> MAEHRIPVLLLLVVVAASSLAQQIPLQKHYIIYEVRNIEKTPEEVKEEMKDTDILYSFKALGAPSYHIVVEVNPRNMRKLEEVELKGKIRMVPVVNMVDVAETLGVSWPRSGARLLDVNLTLIERTLNQEGLTSQESEAHLKGFMEELKDRLQQYNYQAFFTIGASPPKMYI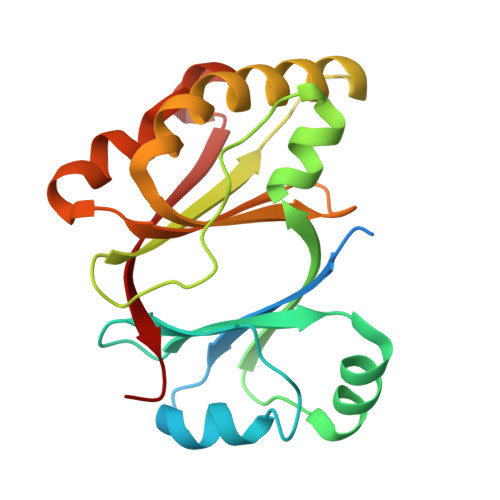YINIPYEEVDKFACIGINQFGGPAAVNTTVSFISSFPK> GMEKLSAIKKPDINVADAWEQYWNKTLVNSTPVLWDANVERAVVVDLPRFELLFNPELPLIDFACGNGTQTKFLSQFFPRVIGLDVSK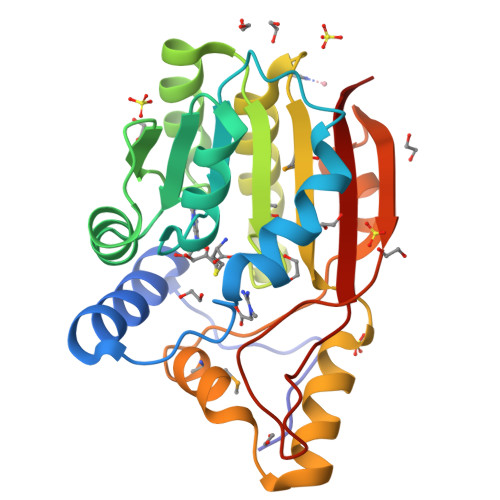SALEIAAKENTAANISYRLLDGLVPEQAAQIHSEIGDANIYMRTGFHHIPVEKRELLGQSLRILLGKQGAMYLIELGTGCIDFFNSLLEKYGQLPYELLLVMEHGIRPGIFTAEDIELYFPDFEILSQGEGLFQSIHKLPDGNYATPPAFWAVIKHR1,5-dimethyl-6-(2-oxidanyl-6-oxidanylidene-cyclohexen-1-yl)carbonyl-3-(2-phenylethyl)quinazoline-2,4-dione 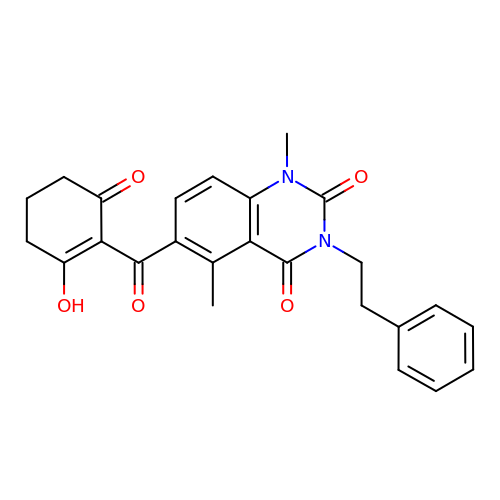| C25 H24 N2 O5 | GZAFFHHHKALSDD-UHFFFAOYSA-N>[2x]MTDNTYQPAKVWTWDKSAGGAFANINRPVSGPTHEKTLPVGKHPLQLYSLGTPNGQKVTIMLEELLALGVTGAEYDAWLIRIGDGDQFSSGFVEVNPNSKIPALRDHTHNPPIRVFESGSILLYLAEKFGYFLPQDLAKRTETMNWLFWLQGAAPFLGGGFGHFYHYAPVKIEYAINRFTMEAKRLLDVLDKQLAQHKFVAGDEYTIADMAIWPWFGNVVLGGVYDAAEFLDAGSYKHVQRWAKEVGER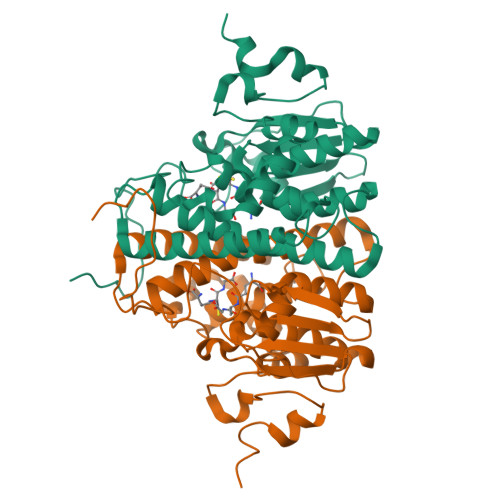PAVKRGRIVNRTNGPLNEQLHERHDASDFETNTEDKRQG>[9x]DITVYNGQHKEAAQAVADAFTRATGIKVKLNSAKGDQLAGQIKEEGSRSPADVFYSEQIPALATLSAANLLEPLPASTINETRGKGVPVAAKKDWVALSGRSRVVVYDT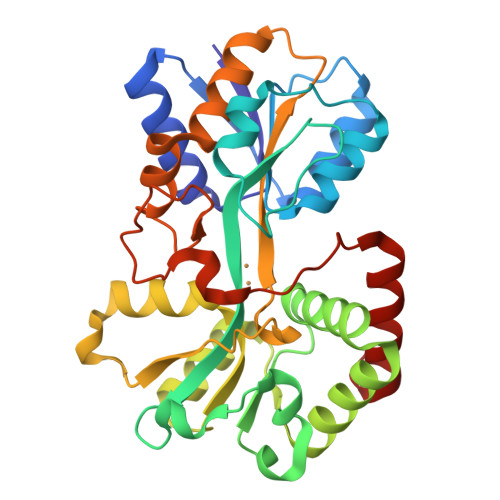RKLSEKDLEKSVLNYATPKWKNRIGYVPTSGAFLEQIVAIVKLKGEAAALKWLKGLKEYGKPYAKNSVALQAVENGEIDAALINNYYWHAFAREKGVQNVHTRLNFVRHRDPGALVTYSGAAVLKSSQNKDEAKKFVAFLAGKEGQRALTAVRAEYPLNPHVVSTFNLEPIAKLEAPQVSATTVSEKEHATRLLEQAGMK>[12x]MTDTNITTPALTADPEVAAAAAQFLTPVVHKMQALVVNGKQAHWNVRGSNFIAIHELLDSVVAHAQDYADTAAERIVALGLPIDSRVSTMAEKTSTAVPAGFAQWQDEIKAIV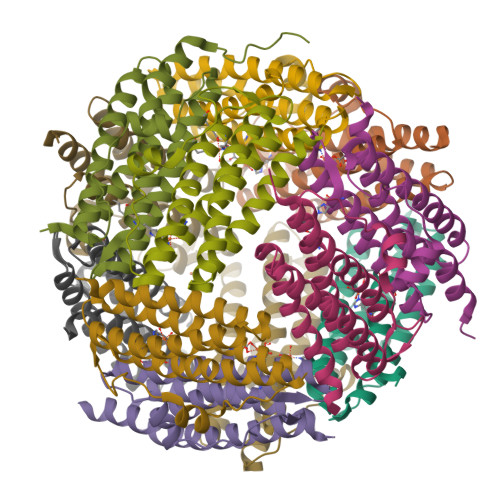SDIDAALVDLQAAIDGLDEVDLTSQDVAIEIKRGVDKDRWFLLAHLAE>PCCEVITNVNLPDDNVQSTLSQIENAISDVMGKPLGYIMSNYDYQKNLRFGGSNEAYCFVRITSIGGINRSNNSALADQITKLLVSNLNVKSRRIYVEFRDC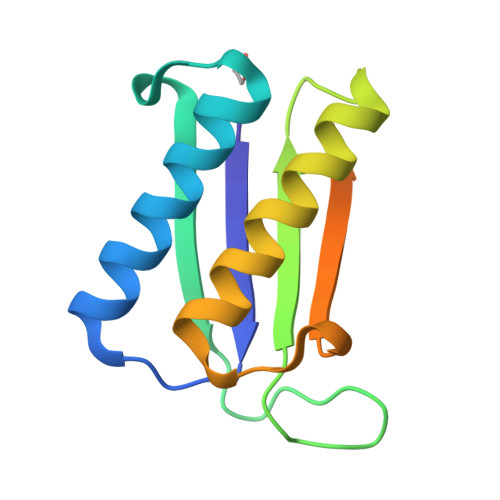SAQNFAFSGSLFGGSRSHHHHHH[2x]> MFRWLFLYWYNSTDTPSAIAKVNLWSYINLRLFKARLSSSIAYYILGLNN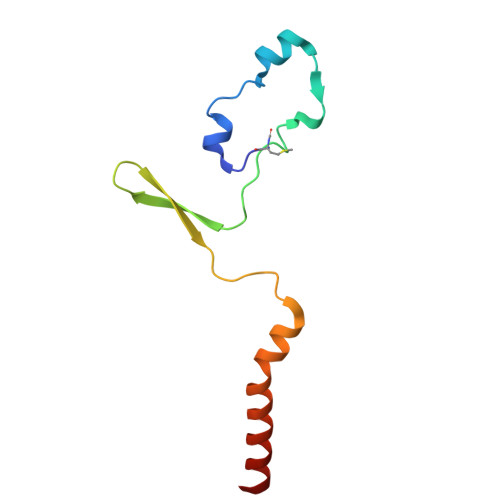LELKKLKIFYKNTYFDYIYLKSIPCLFLIIFFTNLYLFL>[2x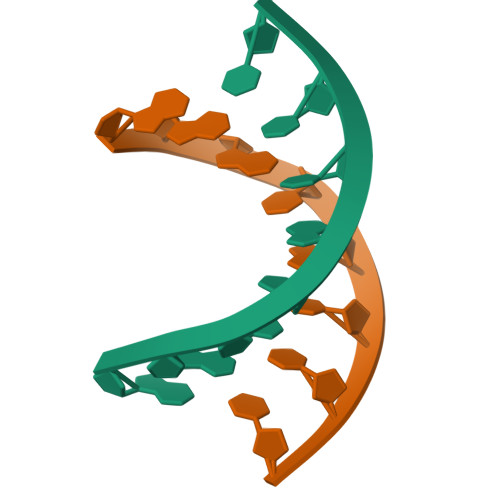]GGGTACCC>HHHHHHSSGLVPRGSHMMSKIKFMRSDLIDEAKEVVQHRTEKEKDTLHETPGIKMKEDRNGRVHITHIDVDESGAESIGKKKGTYITLTVPTLTVEDAQGFQELNQQLISSLKDIHQALMLTDQSKILVIGLGNRTITPDAIGPVAIDRFHEAIFSSPIEFGQVVYYAPGVTGQTGLETGEFVRAISERVKPDLIIVIDALAARNQDRLCKSLQITNTGIHPGSGVGNSRNEISFESLGVPVTAIGVPMVVDAPVLVVEAIETVFKVISSQIGETTKPSSALSVGPWLRSTDEPINVDAIKPIFGEWTAWSSEELHALLDEVLPPRHQQLF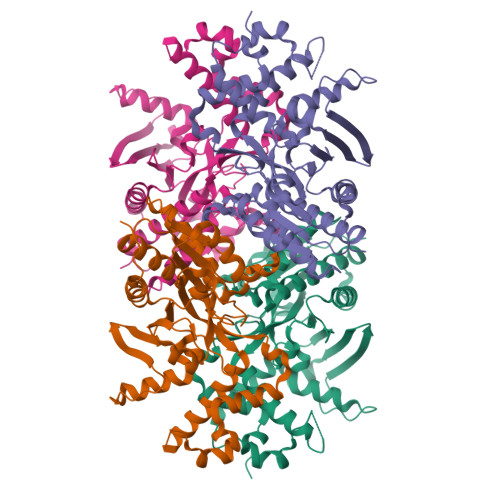VTPKESDAWVIMHADLIQTGILNWLQDDVFGSISP[2x]>MGSDKIHHHHHHMIYYGTMFDHKVRFSIVRMREVVEEARNRHALSYLATVVLGRALIGAALVTPWLAEKERWTLDIEGNGPIRRVVAQSTS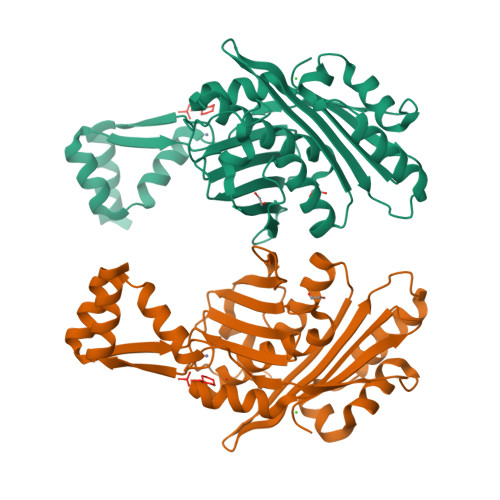EFTVRGYVANPKVELPLNEKGKFDVAGAIGQGVLRVVRDLGLKTPFVSQVPLVSGEIAEDLAYYFAVSEQIPSAFSIGVLVDSDGVKIAGGFAVQIIDRTLEQEKVEMIEKNIKNLPSISKLFQEAEPLDVLERIFGEKVGFVETAEIKYKCDCNREKAKNALLVLDKKELEDMRKEGKGEVVCKWCNTRYVFSEEELEELLKFKVDDSGS[2x]> TLDGPYQPTSLNLPVDYWMLIAPTREGKVAEGTNTTDRWFACVLVEPNVQN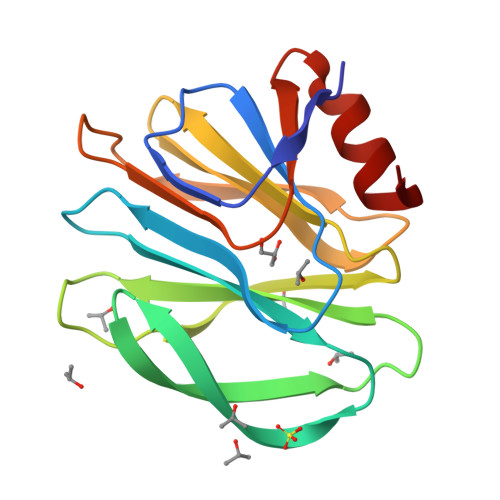TQRQYVLDGQNVQLHVSNDSSTSWKFILFIKLTPDGTYTQYSTLSTPHKLCAWMKRDNRVYWYQGATPNASESYYLTINNDNSNVSSDAEFYLIPQSQTAMCTQYINNGL>MHHHHHHTSKIEQPRWASKDSAAGAASTPDEKIVLEFMDALTSNDAAKLIEYFAEDTMFQAMPLPPAYGRDAVEQTLAGLFTVMSIDAVETFH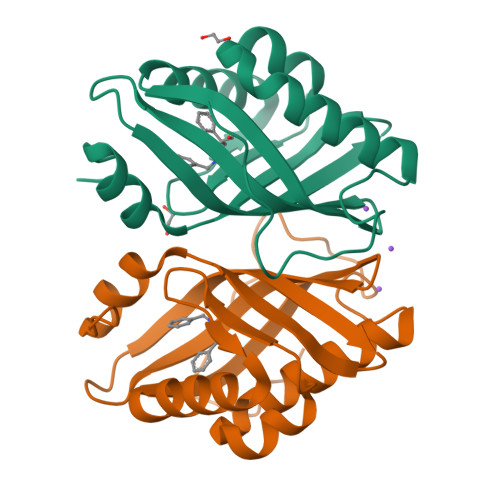IGSSNGLVYTERVDVLRALPTGKSYNLSILGVFQLTEGKITGWRDYFDLREFEEAVDLPLRG[4x]> IEIDVLCDLTQRQAKLYQVLKSQISTNYDAIENAATNDSTSNSASNSGSDQNLINAVMQFRKVCNHPDLFERADVDSPFSFTTFGKTTSMLTASVANNNSSVISNSNMNLSSMSSNNISNGKFTDLIYSSRNPIKYSLPRLIYEDLILPNYNNDVDIANKLKNVKFNIFNPSTNYELCLFLSKLTGEPSLNEFFRVSTTPLLKRVIERTNGPKNTDSLSFKTITQELLEVTRNAPSEGVMASLLNVEKHAYEREYLNCIQRGYHPNVSAPPVTIEVLGSSHVTNSINNELFDPLISQALSDIPAITQYNMHVKKGIPVEDFPKTGLFPEPLNKNFSSNISMPSMDRFITESAKLRKLDELLVKLKSEGHRVLIYFQMTKMMDLMEEYLTYRQYNHIRLDGSSKLEDRRDLVHDWQTNPEIFVFLLSTRAGGLGINLTAADTVIFYDSDWNPTIDSQAMDRAHRLGQTRQVTVYRLLVRGTIEERM;> KAVVIDDPPLRQTPEPFDEQSAYNPQSPIAIDFGSSKLRAGFVNHATPTHIFPNALTKFRDRKLNKNFTFVGNDTLLDQAVRSQSRSPFDGPFVTNWNLTEEILDYTFHHLGVVPDNGIPNPILLTERLATVQSQRTNWYQILFETYNVPGVTFGIDSLFSFYNYNPSGNKTGLVISCGHEDTNVIPVVDGAGILTDAKRINWGGHQAVDYLNDLMALKYPYFPTKMSYLQYETMYKDYCYVSRNYDEDIEKILTLENLDTNDVVVEAPFTEVLQPQKTEEELRIQAEKRKETGKRLQEQARLKRMEKLVQKQEEFEYFSKVRDQLIDEPKKKVLSVLQNAGFDDERDFKKYLHSLEQSLKKAQMVEAEDDSHLDEMNEDKTAQKFDLLDIADEDLNEDQIKEKRKQRFLKASQDARQKAKEEKERVAKEEEEKKLKEQQWRETDLNGWIKDKRLKLNKLIKRRKEKLKLRDEMKDRKSQVSQNRMKNLASLAEDNVKQGAKRNRHQATIDNDPNDTFGANDEDWLIYTDITQNPEAFEEALEYEYKDIVELERLLLEHDPNFTEEDTLEAQYDWRNSILHLFLRGPRPHDSENIHEQHQMHLNVERIRVPEVIFQPTMGGQDQAGICELSETILLKKFGSQPGKLSQTSIDMVNNVLITGGNAKVPGLKERIVKEFTGFLPTGTNITVNMSSDPSLDAWKGMAALARNEEQYRKTVISKKEYEEYGPEYIKEHKLGNTKYFED;> ERLLFLRSVGERNEIGFPSRFKSAHYKKPTRRHKSARQLISDENKRINALLTKANKAAESSTAARRLVPKATYFSVEAPPSIRPAKKYCDVTGLKGFYKSPTNNIRYHNAEIYQLIVKPMAPGVDQEYLKLRGANFVLK;>VTRTAAHTHIKGLGLDESGVAKRVEGGFVGQIEAREACGVIVDLIKAKKMSGRAILLAGGPSTGKTALALAISQELGPKVPFCPLVGSELYSVEVKKTETLMENFRRAIGLRIKETKEVYEGEVTELTPEDAENPLGGYGKTISHVIVGLKSAKGTKTLRLDPTIYESIQREKVSIGDVIYIEANTGAVKRVGRSDAYATEFDLETEEYVPLPKGEVHKKKEIVQDVTLHDLDVANARPQGGQDVISMMGQLLKPKKTEITEKLRQEVNKVVAKYIDQGVAELIPGVLFIDEVNMLDIEIFTYLNKALESNIAPVVVLASNRGMTTVRGTEDVISPHGVPPDLIDRLLIVRTLPYDKDEIRTIIERRATVERLQVESSALDLLATMGTETSLRYALQLLAPCGILAQTSNRKEIVVNDVNEAKLLFLDAKRSTKILETSANYL[3x];>[3x]KSLSLIAAHSHITGLGLDENLQPRPTSEGMVGQLQARRAAGVILKMVQNGTIAGRAVLVAGPPSTGKTALAMGVSQSLGKDVPFTAIAGSEIFSLELSKTEALTQAFRKSIGIKIKEETELIEGEVVEIQIDRSITGGHKQGKLTIKTTDMETIYELGNKMIDGLTKEKVLAGDVISIDKASGKITKLGRSFARSRDYDAMGADTRFVQCPEGELQKRKTVVHTVSLHEIDVINSRTQGFLALFTGDTGEIRSEVRDQINTKVAEWKEEGKAEIVPGVLFIDEVHMLDIECFSFINRALEDEFAPIVMMATNRGVSKTRGTNYKSPHGLPLDLLDRSIIITTKSYNEQEIKTILSIRAQEEEVELSSDALDLLTKTGVETSLRYSSNLISVAQQIAMKRKNNTVEVEDVKRAYLLFLDSARSVKYVQENESQYIDDQGNVQISIAKSADPDAMDTTE;> FVKPRRPYNSEGMTRILRRYEEDLFCTF

Unlike other chromatin remodelers, INO80 preferentially mobilizes hexasomes, which can form during transcription. Here, we report cryogenic-electron microscopy (cryo-EM) structures of endogenously purified S. cerevisiae INO80 bound to a hexasome and a nucleosome. We group subunits of the INO80 complex into four modules: Rvb module (Rvb1/Rvb2), Arp8 module (Arp8/Arp4/Actin/Ies4 and Taf14), Ino80 module (Ino80/Ies2) and Arp5 module (Arp5/Ies6). The Ino80 protein consists of three major regions: the N-terminal domain (NTD), the HSA region (Ino80HSA) and the ATPase domain (Ino80ATPase).

In class 1 of the INO80-hexasome structure, Arp8 engages with the ~35 bp of DNA unwrapped from removal of the H2A-H2B dimer and an additional ~5 bp of flanking DNA. In class 1, the hexasome is almost identical with the unbound hexasome, without detectable additional DNA unwrapping. While the INO80 architecture appears similar to that in the INO80-nucleosome structures, a major difference is that it is rotated ~180° on a hexasome compared to a nucleosome. When INO80 binds to a hexasome, the Arp5/Ies6 regions used in the context of a nucleosome are repurposed for different interactions. We observe that Ino80ATPase engages the hexasome predominantly near SHL −2. The placement of Ino80ATPase near SHL-2 is consistent with how the ATPase subunits of other remodelers bind the nucleosome. A site-specific gap at SHL-2 substantially inhibits INO80’s sliding of hexasomes (~2000 fold) while a gap near SHL-6 does not have a major effect. We further propose that the new contacts made by the Arp5/Ies6 module with the exposed H3-H4 surface provide an anchor allowing the Ino80 motor to efficiently pump DNA through the hexasome.> MAFVVTDNCIKCKYTDCVEVCPVDCFYEGPNFLVIHPDECIDCALCEPECGAQAIFSEDEVPEDMQEFIQLNAELAEVWP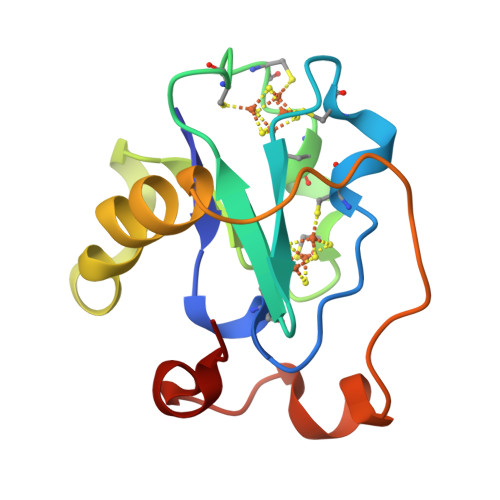NITEKKDPLPDAEDWDGVKGKLQHLER> GGAGCCTGTA;> TACAC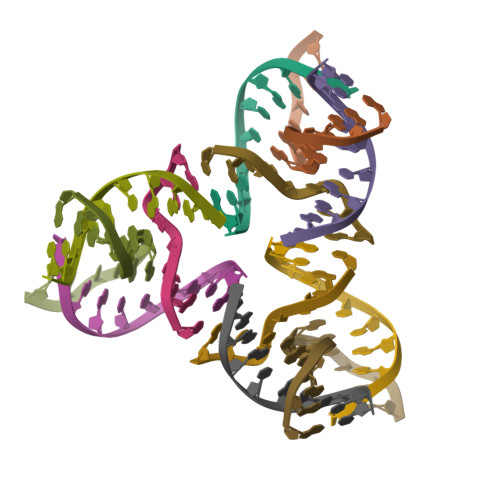CG;> AGACTGTGGCTCC;> CGGACAGTCT>[4x]GPLGSMSQSNRELVVDFLSYKLSQKGYSWSQMAAVKQALREAGDEFELRYRRAFSD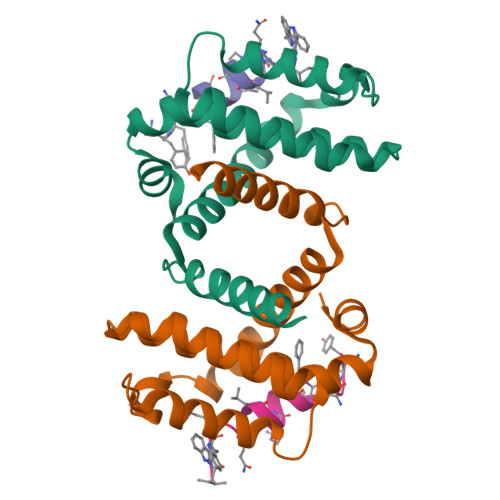LTSQLHITPGTAYQSFEQVVNELFRDGVNWGRIVAFFSFGGALCVESVDKEMQVLVSRIAAWMATYLNDHLEPWIQENGGWDTFVELYGNNAAAESRKGQER;>[4x]IWIAQELRRXGDEXNAYYX> MVAITVQGAQLIKRVVERFYPGIAFNINEGACYIYKFSDHIRRIRMKHGTKYRRQAEEIIRNISLRKERLYGIPVLDEVEWKYVFDGQTFQSYAFEVYVNSILPWSELDPEEEFLRNYRVSREMTEVEKFIEFRAKNEMQIYGDIPIKVWCCFINELSAELKHVPLGMQVMADFVNRFDSPFHQGNRDLSNLEDFQVAYTTPLLFEMCCMESILEFNIKMRMREEEISALEFGDMKVDPVGLLREFFILCLPHPKKINNVLRAPYSWFVKMWGVGADPIVVLQSTAGDDRNSKDVFYDKFRTEPNRYKALFRSSFYNESRRMNEEKILEAVKYSQKLGSHDRRLPLFEKMLKTVYTTPFYPHKSSNMILASFLLSIQTITGYGRAWVKNVSTEFDKQLKPNPSNLVQDVSDLTREFFKQAYVEAKERREEIVKPEDLYTSMLRLARNTSSGFSTEIYVKKRFGPRLRDKDLIKINSRIKALVIFTKGHTVFTDEELHKKYNSVELYQTKGSRDVPIKATRTIYSINLSVLVPQLIVTLPLNEYFSRVGGITSPDYKKIGGKVIVGDLEATGSRVMDAADCFRNSADRDIFTIAIDYSEYDTHLTRHNFRTGMLQGIREAMAPYRDLRYEGYTLEQIIDFGYGEGRVANTLWNGKRRLFKTTFDAYIRLDESERDKGSFKVPKGVLPVSSVDVANRIAVDKGFDTLIAATDGSDLALIDTHLSGENSTLIANSMHNMAIGTLMQREVGREQPGVLTFLSEQYVGDDTLFYTKLHTTDTKVFDKVAASIFDTVAKCGHEASPSKTMMTPYSVEKTQTHAKQGCYVPQDRMMIISSERRKDIEDVQGYVRSQVQTMITKVSRGFCHDLAQLILMLKTTFIGAWKMKRTIKEDAMYRDRKFDSNDEDGFTLIQIRNPLALYVPIGWNGYGAHPAALNIVMTEEMYVDSIMISKLDEIMAPIRRIVHDIPPCWNETQGDKRGLISATKMSFFSKMARPAVQAALSDPQIINLVEELPLGEFSPGRISRTMMHSALLKESSARTLLSSGYELEYQKALNSWITQVSMRLGEESGVISTSYAKLFDVYFEGELDGAPHMFPDQNLSPQFYIQ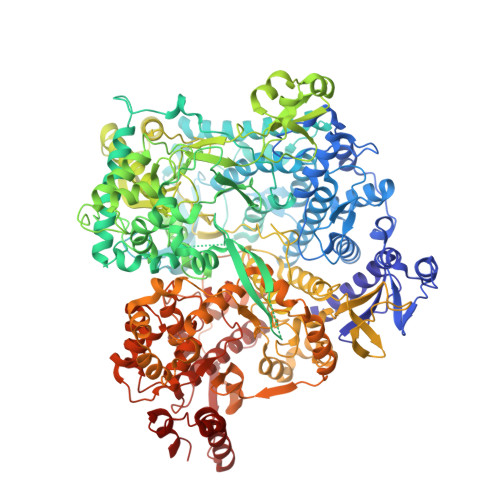KMMIGPRVSSRVRNSYVDRIDVILRKDVVMRGFITANTILNVIEKLGTNHSVGDLVTVFTLMNIETRVAEELAEYMTSEKIRFDALKLLKKGIAGDEFTMSLNVATQDFIDTYLAYPYQLTKTEVDAISLYCTQMIMLRAALGLPKKKMKIVVTDDAKKRYKIRLQRFRTHVPKIKVLKKLIDPNRMTVRNLENQFV Here, we identify functional heterotrimeric G-protein subunits in Entamoeba histolytica, constituting a signaling pathway which, when perturbed, is seen to regulate multiple cellular processes required for pathogenesis. Like mammalian counterparts, EhGα1 forms a heterotrimer with EhGβγ that is dependent on guanine nucleotide exchange and hydrolysis. Despite engaging a classical G-protein effector, EhRGS-RhoGEF, EhGα1 diverges from mammalian Gα subunits and cannot be classified within mammalian Gα subfamilies, as highlighted by distinct structural features in our crystal structure of EhGα1 in the inactive conformation. Here we demonstrate that functional heterotrimeric G-protein subunits are encoded by the pathogen Entamoeba histolytica, including single Gα and Gβ subunits, and two Gγ subunits.

To gain better insight into the distant homology of EhGα1 versus other Gα subunits, we determined a crystal structure of EhGα1 bound to GDP by single-wavelength anomalous dispersion (SAD) using data to 2.6 Å resolution. EhGα1 features the highly conserved Ras-like and all-helical domain structure and nucleotide-binding pocket characteristic of Gα subunits. The three switch regions are ordered in one of the two monomers in the asymmetric unit, likely due to crystal contacts. EhGα1 exhibits a highly conserved mode of nucleotide interaction, including the dispositions of residues Ser-37 and Gln-189. The guanine ring is embraced by the conserved NKxD motif (residues 254–257), with the hydrophobic portion of Lys-255 packing against the planar guanine ring. The phosphate-binding loop (P-loop) forms numerous polar contacts with the α- and β-phosphoryl groups of GDP. Unique to EhGα1 is the absence of an αB helix in the all-helical domain. Although the segment between αA and αC (αA-αC loop) could be affected by crystal packing, five prolines scattered throughout this loop (positions 84, 89, 99, 103, and 106) suggest this region likely also lacks helical structure in solution. EhGα1 also harbors a unique 16-residue insert in the Ras-like domain following the α4 helix. A portion of this insert forms a short β-strand (here termed β7) that extends the six-stranded β-sheet common to all heterotrimeric and Ras-family GTPases, followed by a 15-residue loop that is disordered in our crystal structure.

>SNAKPITVMLLGSGESGKSTIAKQLKILFGGGFPEQERATHKSSICSNVVTCMRTLIEQSAILNHPMKYQPKSKEFTTEDPVTLPFSPELVGDVEALWADEGIQATYEESAKFQLPDCAKYLFENVKRIAMEDYVPTEEDLIHNRTKTTGIHEYDFVVKDIPFHLIDVGGQRSERKKWVSFFSDVDCAIFVTSLAEYDMKLYEDGNTSRLTESIAVFKDIMTNEFLKGAVKLIFLNKMDLFEEKLTKVPLNTIFPEYTGGDNAVMGAQYIQQLFTGKLQTEEMNISGADGTANIEGAVNEKVYTNPTNATDGSNIKRVFMLAVDVIMKNMAANGKMRPTK[2x]> 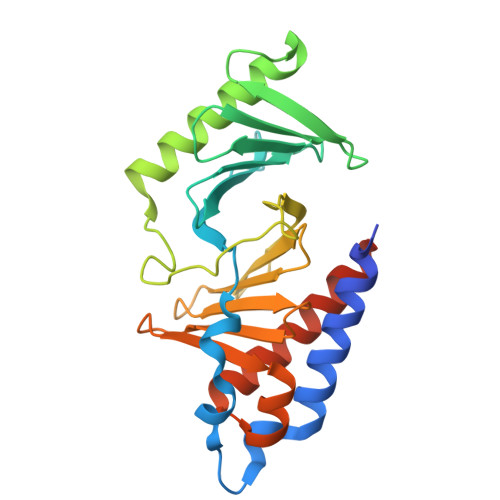RSMETGEVVDCHLSDMLQQLHSVNASKPSERGLVRQEEAEDPACIPIFWVSKWVDYSDKYGLGYQLCDNSVGVLFNDSTRLILYNDGDSLQYIERDGTESYLTVSSHPNSLMKKITLLKYFRNYMSEHLLKAGANITPREGDELARLPYLRTWFRTRSAIILHLSNGSVQINFFQDHTKLILCPLMAAVTYIDEKRDFRTYRLSLLEEYGCCKELASRLRYARTMVDKLLSSRSASNRLKAS> GNDTAVGGEGSLPIPVSQPHIKMVSELIRISGKNLNEPQMNGSWHYNCNFTFKNTLNKEVTISMAFPFPINDGNSEIALPAGQQTNVGQALVYDFLVTVNDKQVSAQRGNIAPDQNKGLYYEDAYFWKTTFPPLATVNIHHDYSTGATYDVMGYHWVRYVLKTGALWQDSSIG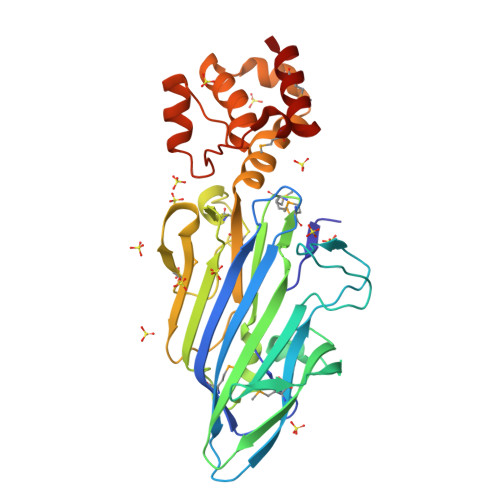HTRLEVIPNTPTRLCSEIDQKADYLNPTPSGMSISGSRADRKYIWDLRHFQPQADLSLCLFTGISYVRYKVIYPWLNSDDALSKLARLSNKELRFLRNTIYAQYGRQFQSPDLQEYFSKKWWYVPNPDYSDRMLNEEDKKLLSMINQAK>TYQYNMNFEKLGKCIIINNKNFDKVTGMGVRNGTDKDAEALFKCFRSLGFDVIVYNDCSCAKMQDLLKKASEEDHTNAACFACILLSHGEENVIYGKDGVTPIKDLTAHFRGDRCKTLLEKPKLFFIQACRGTELADGIQADSRYKIPVEADFLFAYSTVPGYYSWRSPGRGSWFVQALCSILEEHGKDLEIMQILTRVNDRVARHFESQS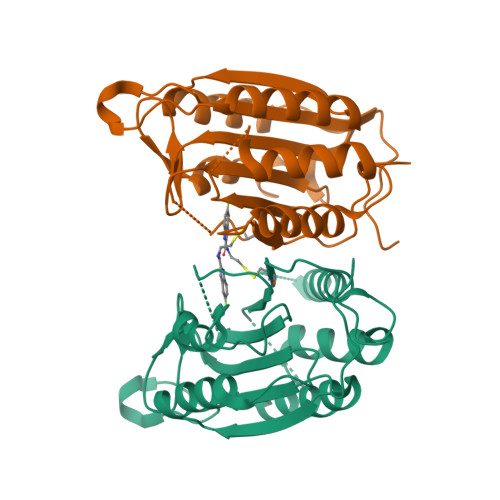DDPHFHEKKQIPCVVSMLTKELYFSQQLHHHHHH[2x]>[4x]MKMEARQKQNSFTSKMQKIVNHRAFTFTVIALILFNALIVGIETYPRIYADHKWLFYRIDLVLLWIFT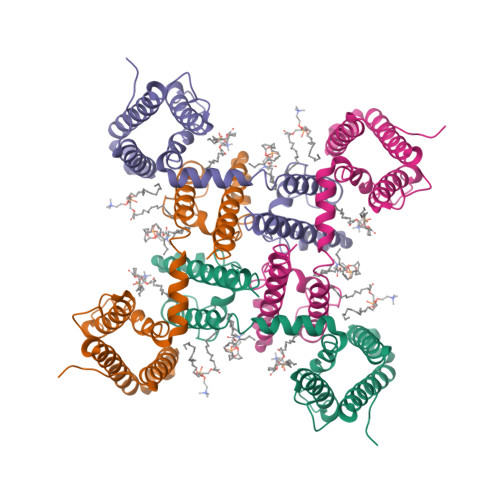IEIAMRFLASNPKSAFFRSSWNWFDFLIVTLSLVELFLADVEGLSVLRILRVLRVLRAISVVPSLRRLVDALVMTIPALGNILILMSIFFYIFAVIGTMLFQHVSPEYFGNLQLSLLTLFQVVTLESWASGVMRPIFAEVPWSWLYFVSFVLIGTFIIFNLFIGVIVNNVEKAELTDNEEDGEADGLKQEISALRKDVAELKSLLKQSK> MKYILFATAGHVDHGKTTLIKTLTGIDTDRLPEEKKRGLSIDIGFAYIDFPDINTRLEIIDVPGHERFIKNAIAGICSASGLILVVDPNEGIMPQTIEHLRVAKSFGIKHGIAVLTKMDKVDEELAHIAEEELIAFLEKEEMNMEIVKVSAVTGQGIEDLKNSIKKLLESINNLNKHKPLRIFVDSAFVVKGYGTVLRGSCFEGEVKEGDKVVVEPIGVISRVRKMQNHGVFVKKAVAGERIALNLPEVDAKKVKRGFLILK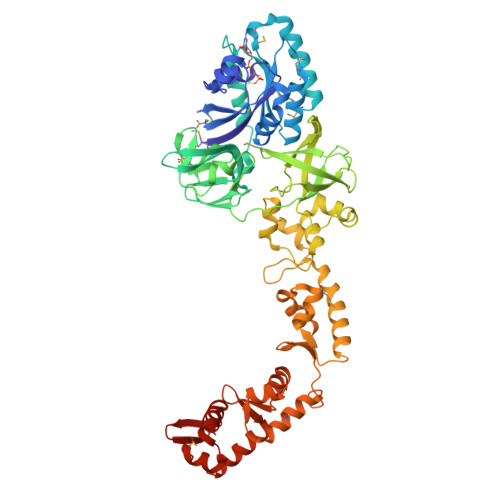PESYEKSNVLIVKTEIDLKPGKIYQVFFGMRETVGKISVIDKGIYLVRLKENAIVRRGDKLVVLDSSGNFLGGAEVLHPKVRVTKKAFIKKNIKDLLENFECYLLKERGPIGLKLEFFKRITGVSPKVANLKPESIEIRGVYYLKGFIENLKLKIKKFLDTELQNAFGVDKEKVKSMFSLNEELLKYILDELKTYKIVNELIIDERKSDLEKNEDFQKLMSILKGGIKEEREIILEGIPKEILTLSIKRKYAHRIGEYLIISDELLKKYINELKELGKTFNVQQAKNKLGLTRKYLIPLLEYLDYLGLTVREGNERRWKR>MPVDRILEAELAVEQKSDQGVEGPGGTGGSGSSPNDPVTNICQAADKQLFTLVEWAKRIPHFSSLPLDDQVILLRAGWNELLIASFSHRSIDVRDGILLATGLHVHRNSAHSAGVGAIFDRVLTELVSKMRDMRMDKTELGCLRAII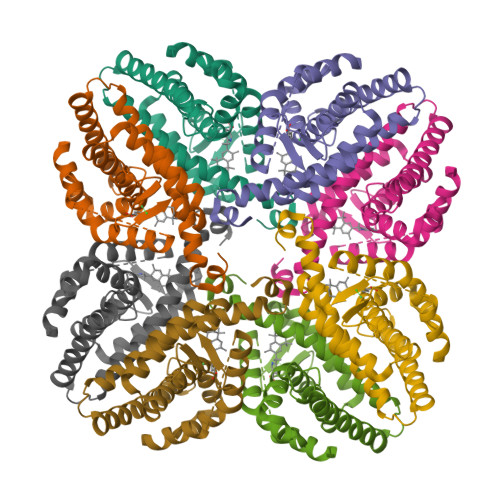LFNPDAKGLSNPSEVEVLREKVYASLETYCKQKYPEQQGRFAKLLLRLPALRSIGLKCLEHLFFFKLIGDTPIDTFL[4x]>[3x]GYDKDLCEWSMTADQTEVETQIEADIMNIVKRDRPEMKAEVQKQLKSGG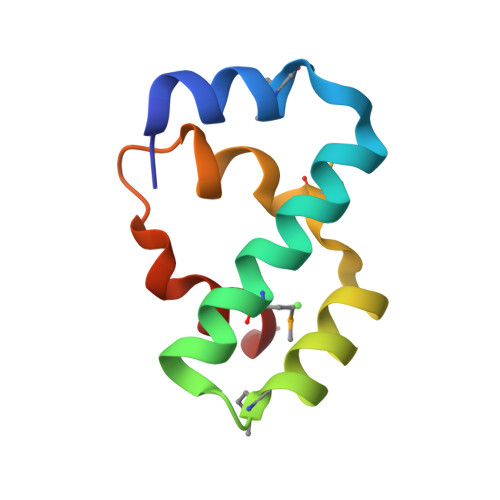VMQYNYVLYCDKNFNNKNIIAEVVGE> NVEEETKYIELMIVNDHLMFKKHRLSVVHTNTYAKSVVNMADLIYKDQLKTRIVLVAMETWATDNKFAISENPLITLREFMKYRRDFIKEKSDAVHLFSGSQFESSRSGAAYIGGICSLLKGGGVNEFGKTDLMAVTLAQSLAHNIGIISDKRKLASGECKCEDTWSGCIMGDTGYYLPKKFTQCNIEEYHDFLNSGGGACLFNKPSKLLD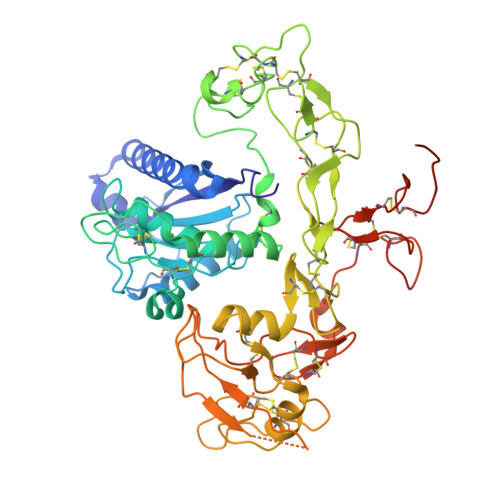PPECGNGFIETGEECDCGTPAECVLEGAECCKKCTLTQDSQCSDGLCCKKCKFQPMGTVCREAVNDCDIRETCSGNSSQCAPNIHKMDGYSCDGVQGICFGGRCKTRDRQCKYIWGQKVTASDKYCYEKLNIEGTEKGNCGKDKDTWIQCNKRDVLCGYLLCTNIGNIPRLGELDGEITSTLVVQQGRTLNCSGGHVKLEEDVDLGYVEDGTPCGPQMMCLEHRCLPVASFNFSTCLSSKEGTICSGNGVCSNELKCVCNRHWIGSDCNTYFPHNDDAKTGITLSG~{N}-[[6-[(cyclohexylmethylamino)methyl]imidazo[1,2-a]pyridin-2-yl]methyl]-4-oxidanylidene-1~{H}-pyrido[1,2-a]pyrimidine-2-carboxamide 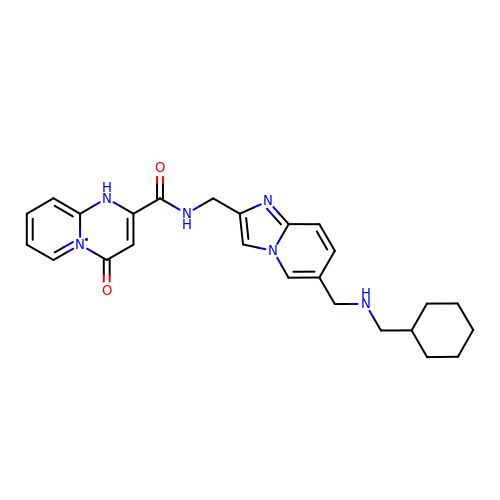| C25 H29 N6 O2 | SUWOYRGBAIBWQL-UHFFFAOYSA-N>GSHMLGKIMLNYTKNIRAAAAQISPVLFSQQGTMEKVLDAIANAAKKGVELIVFPETFVPYYPYFSFVEPPVLMGKSHLKLYQEAVTVPGKVTQAIAQAAKTHGMVVVLGVNEREEGSLYNTQLIFDADGALVLKRRKITPTYHERMVWGQGDGAGLRTVDTTVGRLGALACWEHYNPLARYALMAQHEQIHCGQFPGSMVGQIFADQMEVTMRHHALESGCFVINATGWLTAEQKLQITTDEKMHQALSGGCYT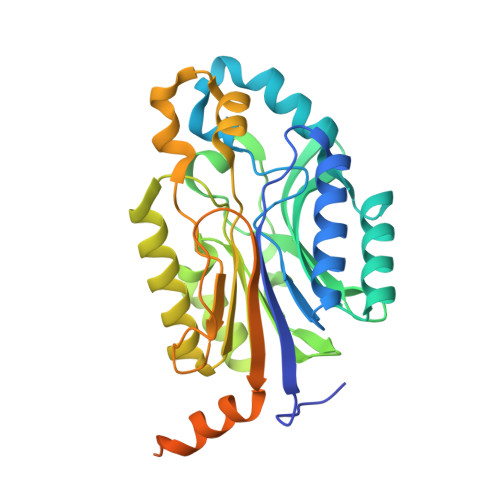AIISPEGKHLCEPIAEGEGLAIADLDFSLIAKRKRMMDSVGHYARPDLLQLTLNNQPWSALEANPVTPNAIPAVSDPELTETIEALPNNPIFSH[2x]>AVVASLKPVGFIASAIADGVTETEVLLPDGASEHDYSLRPSDVKRLQNADLVVWVGPEMEAFMQKPVSKLPGAKQVTIAQLEDVKPLLMKSIHGDDDDHDHAEKSDEDHHHGDFNMHLWLSPEIARATAVAIHGKLVELMPQSRAKLDANLKDFEAQLASTETQVGNELAPLKGKGYFVFHDAYGYFEKQFGLTPLGHFTVNPEIQPGAQRLHEIRTQLVE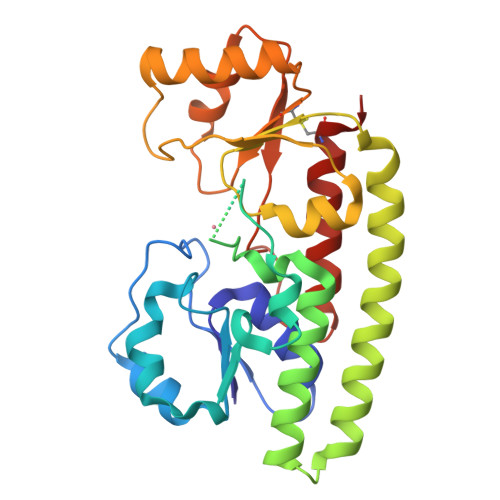QKATCVFAEPQFRPAVVESVARGTSVRMGTLDPLGTNIKLGKTSYSEFLSQLANQYASCLKGD[2x]>[2x]MGSMHAALSTEVVHLRQRTEELLRCNEQQAAELETCKEQLFQSNMERKELHNTVMDLRGNIRVFCRIRPPLESEENRMCCTWTYHDESTVELQSIDAQAKSKMGQQIFSFDQVFHPLSSQSDIFEMVSPLIQSALDGYNICIFAYGQTGSGKTYTMDGVPESVGVIPRTVDLLFDSIRGYRNLGWEYEIKATFLEIYNEVLYDLLSNEQKDMEIRMAKNNKNDIYVSNITEETVLDPNHLRHLMHTAKMNRATASTAGNERSSRSHAVTKLELIGRHAEKQEISVGSINLVDLAGSESPKTSTRMTETKNINRSLSELTNVILALLQKQDHIPYRNSKLTHLLMPSLGGNSKTLMFINVSPFQDCFQESVKSLRFAASVNSCKMTKAKRNRYLNNSVANSSTQSNNSGNFDK

Kinesin motor proteins hydrolyze ATP to produce force and do work in cells. Despite their diverse functions, the kinesin proteins contain a common motor domain with highly conserved or invariant sequence motifs that mediate basic motor properties, such as microtubule binding and ATP hydrolysis. For example, kinesin-14 motors move on microtubules towards the minus end instead of the plus end. Here we report a new crystal structure of human kinesin-14 KIFC1, together with new crystal structures of Drosophila Ncd, a KIFC1 orthologue, and human KIFC3, a divergent KIFC1 paralogue, and an analysis of the structural features of the proposed KIFC1 AZ82 inhibitor-binding site.

The new Ncd dimer structure (2.8 Å) was crystallized in the presence of Mg-AMP·PNP, but was refined with Mg-ADP bound to the nucleotide cleft. The dimeric motor shows the stalk and one head, H1, rotated relative to the other head, H2, positioning the two heads asymmetrically with respect to the coiled-coil stalk. The new structure resembles previous mutant Ncd structures that are interpreted to show the motor as it binds to a microtubule in a force-producing conformation. However, this is the first detailed report of wild-type Ncd in a stalk-rotated conformation. As in previous stalk-rotated mutant Ncd structures, the two heads of the new wild-type Ncd structure are thought to represent different states of the motor – H1 shows extensive interactions with the end of the coiled-coil stalk, or neck, while H2 shows disrupted neck interactions and appears positioned to bind to a microtubule. The two heads differ from one another in the conformation of loops L8, L10 and L12, which are ordered in H1, but disordered in H2. Strikingly, Ncd H2 strand β3 has moved upward from its buried position in H1 – it does this by gaining a residue at its C terminus (G434), as well as its N terminus (N427). The transition of G434 to a β-strand in Ncd head H2 β3 shortens the adjacent P-loop by a glycine residue, which may make the P-loop less flexible and more likely to release bound nucleotide. This is consistent with the reduced density of ADP bound to head H2 compared to head H1, supporting the interpretation that head H2 is releasing ADP, representing a microtubule-binding conformation. Loop L13 is thought to mediate stalk rotation in kinesin-14 Ncd: L13 S639 hydrogen bonds to G347D at the end of the stalk in the Ncd G347D mutant, disrupting neck-motor interactions, including N340-K640 – these interactions maintain stalk position relative to the motor domain and when disrupted, the stalk rotates. The new wild-type Ncd crystal structure shows movement of G347 towards L13 S639, as observed in Ncd G347D (see Fig. 4 of ref.32), and disruption of N340-K640 in head H2, indicating that this interaction is also critical in wild-type Ncd.> MFSAGHKIKGTVVLMPKNELEVNPDGSAVDNLNAFLGRSVSLQLISATKADAHGKGKVGKDTFLEGINTSLPTLGAGESAFNIHFEWDGSMGIPGAFYIKNYMQVEFFLKSLTLEAISNQGTIRFVCNSWVYNTKLYKSVRIFFANHTYVPSETPAPLVSYREEELKSLRGNGTGERKEYDRIYDYDVYNDLGNPDKSEKLARPVLGGSSTFPYPRRGRTGRGPTVTDPNTEKQGEVFYVPRDENLGHLKSKDALEIGTKSLSQIVQPAFESAFDLKSTPIEFHSFQDVHDLYEGGIKLPRDVISTIIPLPVIKELY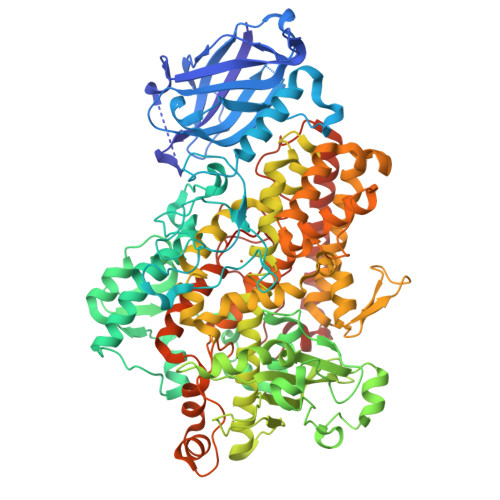RTDGQHILKFPQPHVVQVSQSAWMTDEEFAREMIAGVNPCVIRGLEEFPPKSNLDPAIYGDQSSKITADSLDLDGYTMDEALGSRRLFMLDYHDIFMPYVRQINQLNSAKTYATRTILFLREDGTLKPVAIELSLPHSAGDLSAAVSQVVLPAKEGVESTIWLLAKAYVIVNDSCYHQLMSHWLNTHAAMEPFVIATHRHLSVLHPIYKLLTPHYRNNMNINALARQSLINANGIIETTFLPSKYSVEMSSAVYKNWVFTDQALPADLIKRGVAIKDPSTPHGVRLLIEDYPYAADGLEIWAAIKTWVQEYVPLYYARDDDVKNDSELQHWWKEAVEKGHGDLKDKPWWPKLQTLEDLVEVCLIIIWIASALHAAVNFGNYPYGGLIMNRPTASRRLLPEKGTPEYEEMINNHEKAYLRTITSKLPTLISLSVIEILSTHASDEVYLGQRDNPHWTSDSKALQAFQKFGNKLKEIEEKLVRRNNDPSLQGNRLGPVQLPYTLLYPSSEEGLTFRGIPNSISI> DEYDYLFKVVLIGDSGVGKSNLLSRFTR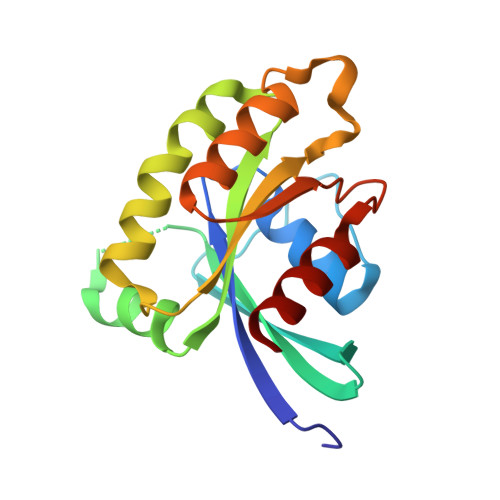NEFNLESKSTIGVEFATRSIQVDGKTIKAQIWDTAGQERYRAITSAYYRGAVGALLVYDIAKHLTYENVERWLKELRDHADSNIVIMLVGNKSDLRHLRAVPTDEARAFAEKNGLSFIETSALDSTNVEAAFQTILTEIY>SNAMIIRPEQHWFLRLFDAHGSVLSKIIFRLLLNVLMSIIAIISYQWYEQLGIHLTVAPFSLLGIAIAIFLGFRNSASYSRFVEARNLWGTVLIAERTLVRQLRNILPAEHDAHRRIVSYLVAFSWSLKHQLRKTDPTADLRRLLPEERVTEILASSMPTNRILLLAGNEIGQLREAGKLSDITYGLMDNKLDELAHVLGGCERLATTPVPFAYTLILQRTVYLFCTLLPFALVGDLHYMTPFVSVFISYTFLSWDSLAEELEDPFGTAANDLPLNAMCNTIERNLLDMTGQHPLPE[5x]

Human bestrophin1 (hBest1) is a Ca2+-activated Cl− channel essential for Cl− transport in retinal pigment epithelium (RPE). Although the structure of hBest1 is still unsolved, two Best1 homolog structures, one from bacteria Klebsiella pneumoniae (KpBest) and the other from chicken (cBest1), have been previously reported. Overall, the channel is a pentameric assembly with a single ion-conducting pathway, which varies in diameter along its length and is constrained at two narrow points: a “neck” contributed by three residues (I62/I66/F70 in KpBest and I76/F80/F84 in hBest1/cBest1) on a transmembrane helix, and an “aperture” formed by a single residue (I180 in KpBest1, I205 in hBest1, and V205 in cBest1) on a cytosolic helix. Here, by electrophysiological and structural analyses, we show that the neck and aperture in hBest1 are both indispensable Ca2+-dependent gates, and their dysregulated opening by rationally designed or patient-derived mutations causes Ca2+-independent leak and elevates Ca2+-dependent channel activity.

Alanine substitution mutants for each of the 12 residues were generated in KpBest and hBest1 and subjected to crystallography and patch clamp, respectively. Moreover, the equivalent KpBest mutants (W16A, G18A, S19A, L259A, P262A, G264A, and D269A) all showed an overall similar structure to that of WT KpBest. The corresponding “Ca2+-binding” sites in WT KpBest are occupied by Zn2+, an essential component in the crystallization buffer. Notably, the short extracellular domains of hBest1 represent a challenge for quantitative measurement of the surface expression by labeling techniques (e.g., biotin). They can be classified into three groups by different molecular mechanisms: (1) mutations on residues involved in Ca2+ binding, including W24A, G26A, S27A, L294A, P297A, F298A, G299A, and D304A, likely cause defects of Ca2+-dependent activation; (2) mutations at the neck/aperture, including I205A, I205T, 3A, and 4A, increase open probability by functionally mimicking a constant open state; and (3) mutations outside of the neck/aperture, including D203A, P233A, Y236A, Y236C, W287A, and W287F, alter open probability through the neck/aperture residues.>[11x]KFSKEQLRTFQMIHENFGRALSTYLSGRLRTFVDVEISIDQLTYEEFIRSVMIPSFIVIFTGDVFEGSAIFEMRLDLFYTMLDIIMGGPGENPPNRPPTEIETSIMRKEVTNMLTLLAQAWSDFQYFIPSIEN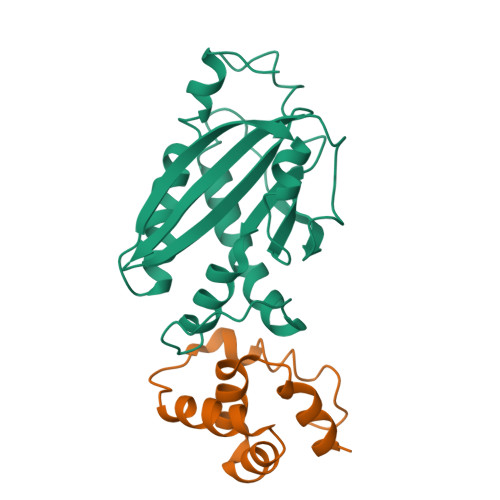VETNPQFVQIVPPNEIVLLVTASVSWGEFTSFINVCWPFSLLEPLLEKLS;>[11x]GSHMVQLVNFLQSEHPQTIAVVLSYLDPPVAAQILGALPEELQTEVLKRIALLERTSPEVVKEIERNLEKKISGF>SMPIILDSDVLEVAEYVYKTRLSQPYTEVGSEWEYNYKNPTATFAKGDGHNLQRYITIDGKQLHRPIHGLAHTMRTLMYSQLMYCSSKKQPSPHVCQDGRTIADLSELDLKKINIAQLFFVAGRESEASYGDAYHRYHLYGAKQFEEYARKH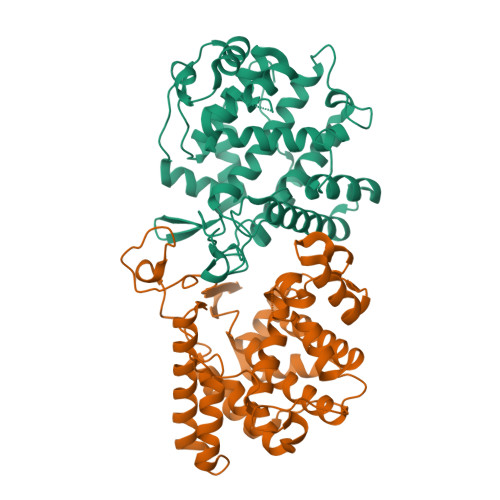LTHLFSEEEIRLYSRCIEDRVGDSFDGTPEGYIIHLSHMIDLMRCKSPVEVFLGHSKGVSGIVPTLIHLFGKQDGLDIMHYARGLFAATGEAVPYIDSSEWPHLGVDLSRVQRALSIVGDINVPGQEADSKKTAQAGFSVDGCYSALTSVPTPSWYEKELKEIDDEKIDVKEVDDREIEKEHEIVVPSQATTPLSTVKTDSFVEKLLKPFMIWKKPEVQTTQPTTEKTNKP[2x]Rab27A and Rab27B are secretory Rabs with well-characterised roles in transport and docking of secretory vesicles (exosomes) at the plasma membrane. Rab27A promotes the growth and invasion of multiple cancer types such as breast, lung and pancreatic, by enhancing secretion of chemokines, metalloproteases and exosomes. Reported co-crystal structures show that several effectors of Rab27A interact with the Rab27A SF4 pocket (‘WF-binding pocket’) via a conserved tryptophan–phenylalanine (WF) dipeptide motif. To obtain structural insight into the ligandability of this pocket, a novel construct was designed fusing Rab27A to part of an effector protein (fRab27A), allowing crystallisation of Rab27A in high throughput.

Covalent ligands are increasingly used to target challenging proteins. fRab27A contains two cysteine residues (C123 and C188) in close proximity to the WF-binding pocket, which are mutated to serine in crystal structures. Sequence alignment of Rab27A and Rab27B against the Rab family demonstrated that these two cysteine residues are unique to Rab27 among other family members (Fig. 1C and S4†), suggesting that cysteine-reactive covalent fragments targeting the WF binding site may offer a means to ligand Rab27 selectively over other Rabs. Compounds A01 and B01 were confirmed as hits against fRab27A-C188 and fRab27A-C123, respectively. Hit fragment A01 preferentially reacted with fRab27A-C188, whereas fragment B01 was found to react with both fRab27A-C123 and fRab27A-C188 with significant rate enhancement over GSH. The phenyl ring of A01 formed an edge-on π-stacking interaction with Y122, which is known to be important for Rab27A-effector interaction, along with hydrophobic interactions with M93 and M185. Residues K11 and D91 were located in close proximity to the methyl ether moiety, suggesting a route to build further polar contacts in analogues of A01. However, in contrast to the fRab27A-C188-A01 structures, in which the SF4 pocket is largely unperturbed by C188 modification, and the Rab27A-Slp2a complex, C123 modification by B01 caused the side chain of Y122 to adopt an alternate conformation, opening up an enlarged cavity in the pocket.

>[2x]HMSFLTEEEQEAIMKVLQRDAALKRAEEERGSGSGSGMSDGDYDYLIKFLALGDSGVGKTSVLYQYTDGKFNSKFITTVGIDFREKRVVYRASGPDGATGRGQRIHLQLWDTAGLERFRSLTTAFFRDAMGFLLLFDLTNEQSFLNVRNWISQLQMHAYSENPDIVLCGNKSDLEDQRVVKEEEAIALAEKYGIPYFETSAANGTNISQAIEMLLDLIMKRMERCVDKS>GSHMASPAPVDLGRAGDFVILAKSGISTSGATHVTGDIGVSPIDRTGLTGFSETMDPSNTFSTSTYVVAPGKLYAADYADPTPAKLTTAVSAMEAAYTDAGGRTGGLSVPGAGTILPATTLPAGVYTWSTGVTIPTGVTLEGGPDDV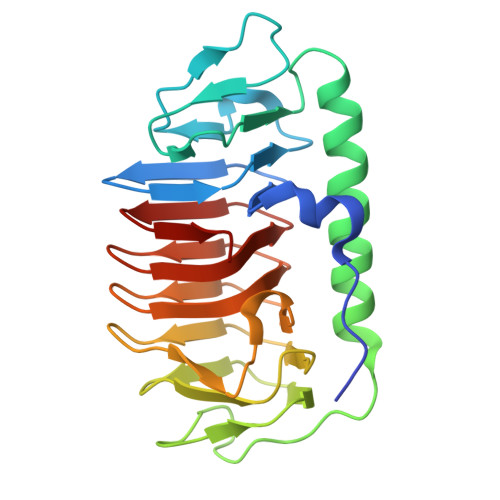WIFQIAGTLDIATDMQVLLKGGAQAKNIFWQVGDVVTLHAGSHFEGNILGFSTIAMQTGASINGKLLSQKEVTLLGSDILTPAP[3x]The polyamine known as spermidine is typically made by spermidine synthase, but in many bacterial species, including 70% of human gut microbes, carboxyspermidine decarboxylase (CASDC) performs the terminal step in the production of spermidine. Carboxyspermidine dehydrogenase is the first enzyme in the pathway and uses NADPH to perform a reductive condensation of aspartate semialdehyde and putrescine (1,4-diaminobutane) to produce carboxyspermi­dine. Carboxyspermidine decarboxylase (CASDC) is a pyridoxal 5′-phosphate (PLP)-dependent enzyme that removes the carboxylate of carboxyspermidine to produce spermidine. CASDC is a homodimer, with each monomer composed of two domains: a β/α-barrel pyridoxal 5′-phosphate-binding domain that forms most of the active site and a β-barrel domain that extends the dimeric interface and contributes to the active site of the opposing monomer.

Here, we report a 1.41 Å resolution X-ray structure of CASDC from Clostridium leptum (ClCASDC), a member of the human gut flora. Electron density corresponding to PLP was observed in the active site of both monomers of ClCASDC. His170 forms a π-stacking interaction with the pyridoxamine ring and Glu237 forms a hydrogen bond to the pyridoxamine nitrogen. Electron density for two conformations of Cys306 was visible. The sulfhydryl group faces away from PLP with 70% occupancy (both chains), placing the sulfur in a position in which it is unable to hydrogen-bond to any surrounding residues. The explanation for this seemingly unfavourable position may lie with the Cys306 backbone carbonyl, which appears to shift ∼1.4 Å between the two conformations. This shift alters the ability of the carbonyl oxygen to donate electrons to the pyridoxamine oxygen and Schiff-base nitrogen, which may be important to facilitate the expected proton transfer during the catalytic cycle. ClCASDC was purified using a N-terminal hexahistidine affinity tag, and electron density for eight residues of this tag was resolved during refinement. The tags appear to originate from the N-terminus of the same monomer, but the linker density is weak and could not be modelled, so the histidine tags were designated chains C and D in the PDB file.

>[2x]MELPFSSLQTPCYVVDEALLERNLVILKQVIDRTGCKILLAQKAFSMFACYPLIGSYLNGTTASGLFEARLGKEEMGGETHIFSPAYREDEIDEILSLCDHVIFNSFSQWEKYKAKVLASGKSAGLRLNPEHSTQDHAIYDPCSPGSRLGITLKKFRPDLLDGIEGLHFHTLCEQDAAPLVETVAVVEEKFGPWLSQMKWLNFGGGHHITRPGYDIDALVSCVSRVQERYGVQVYLEPGEAVALNAGFLVSTVLDVLENSGNIAVLDTSAACHMPDVLEMPYRPPIAGGGGLGEKAYDYRLGGPTCLAGDVIGDYSFDEPLSPGSRVVFCDMAIYSMVKNNTFNGMNLPAIYLKKQDGSIQLVRKFGYEDFKTRLS;>[2x]HHHSSGLV> MGKIATKYHGDIEIHEKDIVRFEQGIPGFLEEKQFVLLQLEDTPFIILQSVNTPALGFVL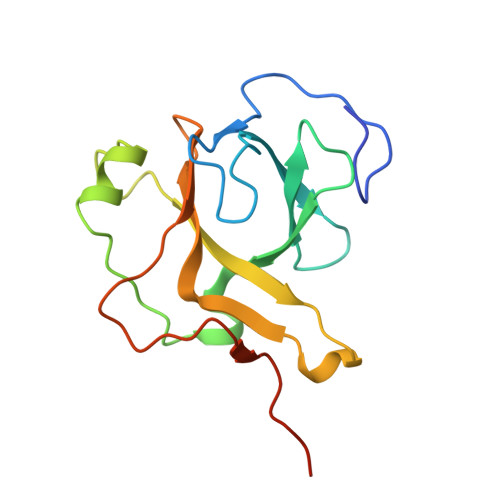IEPFSYFPTYEIDLDDNTLEQLQITGEQDVALYVILTVADPFDDTTANLQAPIVINVHKRLGKQVILTNTNYKTKHRLFPEKVAKHHHHHH> CGRG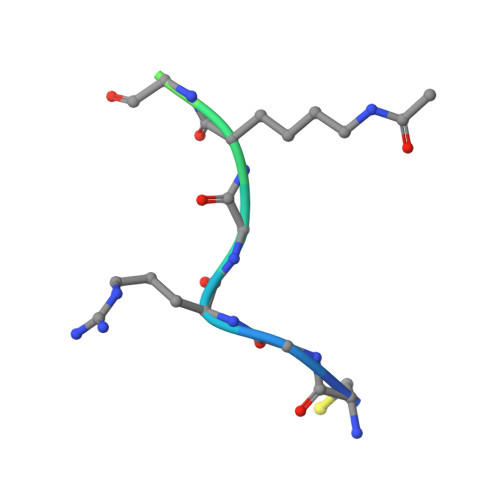KGGKGLGKGGA N-{1-BENZYL-4-[2-(2,6-DIMETHYL-PHENOXY)-ACETYLAMINO]-3-HYDROXY-5-PHENYL-PENTYL}-3-METHYL-2-(2-OXO-TETRAHYDRO-PYRIMIDIN-1-YL)-BUTYRAMIDE 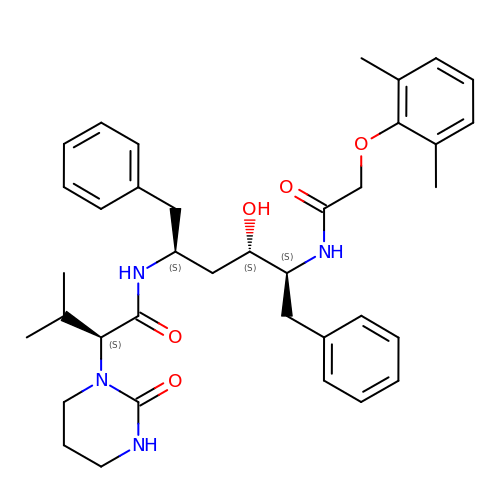| C37 H48 N4 O5 | KJHKTHWMRKYKJE-SUGCFTRWSA-N>NLSQLSFHRVDQKEITQLSHLGQGTRTNVYEGRLRVEGSGDPEEGKMDDEDPLVPGRDRGQELRVVLKVLDPSHHDIALAFYETASLMSQVSHTHLAFVHGVCVRGPENIMVTEYVEHGPLDVWLRRERGHVPMAWKMVVAQQLASALSYLENKNLVHGNVCGRNILLARLGLAEGTSPFIKLSDPGVGLGALSREERVERIPWLAPECLPGGANSLSTAM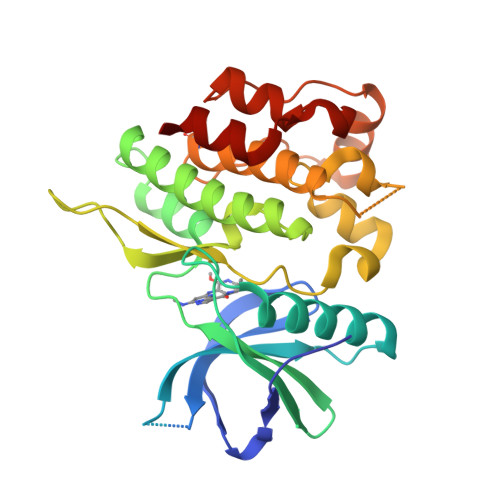DKWGFGATLLEICFDGEAPLQSRSPSEKEHFYQRQHRLPEPSCPQLATLTSQCLTYEPTQRPSFRTILRDLTRL[3x]> MPEGPELHLASQFVNEACRALVFGGCVEKSSVSRNPEVPFESSAYRISA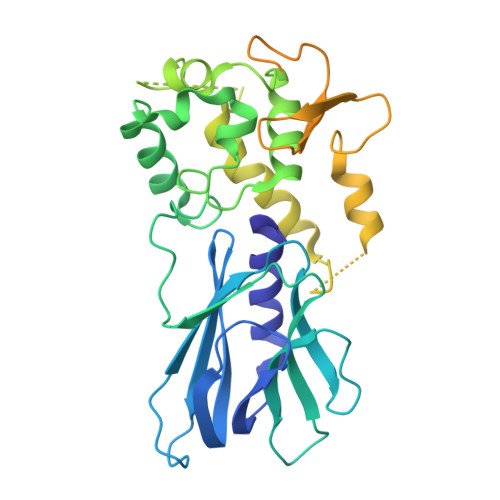SARGKELRLILSPLPGAQPQQEPLALVFRFGMSGSFQLVPREELPRHAHLRFYTAPPGPRLALCFVDIRRFGRWDLGGKWQPGRGPCVLQEYQQFRENVLRNLADKAFDRPICEALLDQRFFNGIGNYLRAEILYRLKIPPFEKARSVLEALQQHRPSPELTLSQKIRTKLQNPDLLELCHSVPKEVVQLGGKGYGSESGEEDFAAFRAWLRCYGMPGMSSLQDRHGRTIWFQGDPGPLAPKGRKSRKKKSKATQLSPEDRVEDALPPSKAPSRTRRAKRDLPKRTATQRPEGTSLQQDPEAPTVPKKGRRKGRQAASGHCRPRKVKADIPSLEPEGTSAS>KTVIKNETGTISISQLNKNVWVHTELGSFNGEAVPSSGLVLNTSKGLVLVDSSWDDKLTKELIEMVEKKFQKRVTDAIITHAHADRIGGIKTLKERGIKAHSTALTAELAKKNGYEEPLGDLQTVTNLKFGNMKVETFYPGKGHTEDNIVVWLPQYNILVGGCLVKSTSAKDLGNVADAYVNEWST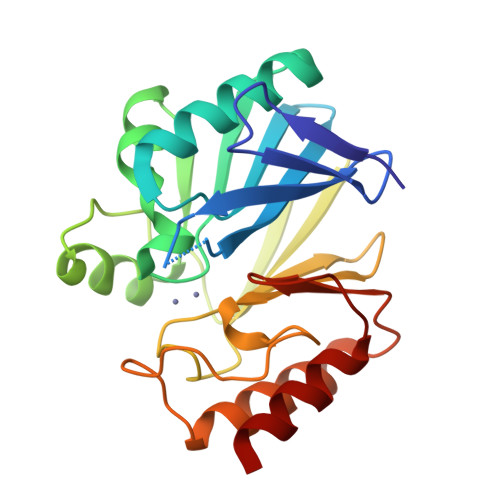SIENVSKRYRNINAVVPSHGEVGDKGLLLHTLDLLK[2x]1(R)-1-ACETAMIDO-2-(3-CARBOXYPHENYL)ETHYL BORONIC ACID | C11 H14 B N O5 | 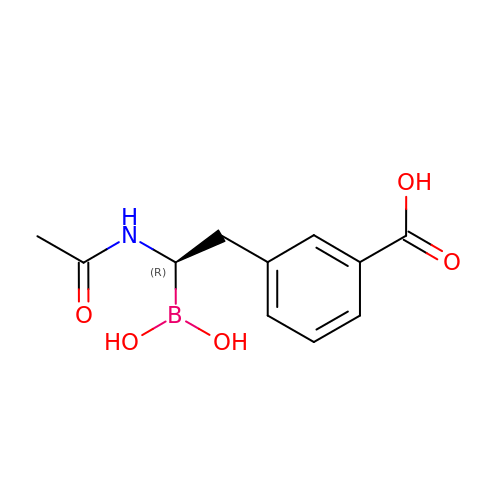OBZSRKUYUGJGIM-JTQLQIEISA-N>MEGLNLVATALAVGLGAIGPGVGIGIIVSGAVQAIGRNPEIENRVVTYMFIGIAFTEALAIFGLVIAFLIGFGVLQ[10x];>[2x]MSTRTRNILIIVGALIISIASRFFLYTGPPHVEVAAEVIFDGIPGFPITNSFVVAIIIDIFVIALAVAATRNLQMVPRGLQNVMEFILESLYNLFRNINAKYVATAFPLVATIFLFVLFGNWFGLLPGVGSIGVCHEKKEEHAVVDERLALAAPAAPLSSVAAAEGEEIHDTCAAQGKKLVPLFRAPAADLNFTFAIAVISFVFIEYWGFRALGPGYLKKFFNTNGIMSFVGIIEFISELVKPFALAFRLFGNIFAGEVLLVVMAFLVPLLLPLPFYGFEVFVGFIQALIFALLTYAFLNIAVTGHDEEHAH;>[4x]MEALGINPTLFIAQLINF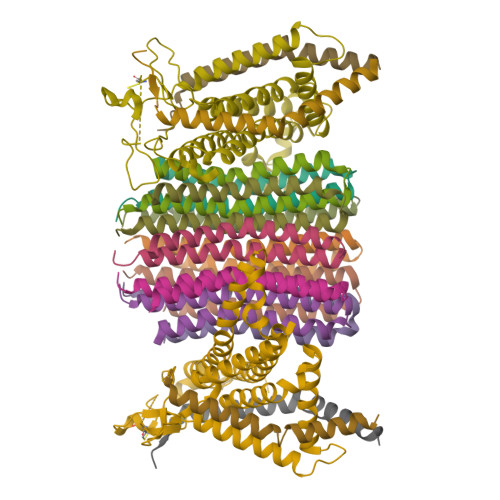LLLIFILRALLYRPVMNLLNERTRRIEESVRDAEKVREQLANARRDYEAEIARARQEAAKIVAQAQERAKQQEAEIIAQARREAERLKEEARAQAEQERIRMLSEAKSQIADLVTLTASRVLGAELQARGHDALIAESLAALDRRN>GPLGSKTKDYKTRDVTDDVKSIVRFVQEHSSSQGMRNIKHVGPSGRFTMNMLVDIFLGSKSAKIQSGIFGKGSAYSRHNAERLFKKLILDKILDEDLYINANDQAIAYVMLGNKAQTVLNGNLKVDFMETENSSSVKKQKALVAKVS[2x]

RecQ helicases, a family of DNA unwinding enzymes that are conserved from bacteria to mammals, play a key role in protecting the genome against deleterious changes (for recent reviews). Mutations in BLM and WRN are associated with the rare genetic diseases Bloom and Werner syndromes, respectively. BLM acts preferentially on recombination and repair intermediates containing HJs to promote efficient branch migration. Novel structural motifs found in the domain, such as the acidic β-wing, the BLM-insertion, and the C-term extended loop, may contribute cooperatively to the specialized functions of BLM in relation to HJ.

Crystals were obtained in conditions that included either a phosphate ion or an arsenate ion. The two crystals, which belong to the same space group, were employed for X-ray data collection. The structures of human BLM RQC complexed with a phosphate ion and an arsenate ion were determined at resolutions of 2.7 and 2.9 Å, respectively. The asymmetric unit of each crystal contains two RQC monomers (Mol-A and -B), which are bridged to each other by the ion (P1 or As1) shared at the interface. These structures demonstrate that P1 and As1 play a key role in lattice formation. Consistently, the phosphate or arsenate ion was a critical determinant of crystallization, and could not be replaced by other salts. For the arsenate ion complex, the X-ray data were also collected at the peak wavelength of arsenate (1.0439 Å) to calculate the anomalous difference Fourier map. The map gave a strong density surrounding the ion, confirming the presence of the arsenate ion in this position.> MGSLVREWVGFQQFPAATQEKLIEFFGKLKQKDMNSMTVLVLGKGGVGKSSTVNSLIGEQVVRVSPFQAEGLRPVMVSRTMGGFTINIIDTPGLVEAGYVNHQALELIKGFLVNRTIDVLLYVDRLDVYAVDELDKQVVIAITQTFGKEIWCKTLLVLTHAQFSPPDELSYETFSSKRSDSLLKTIRAGSKMRKQEFEDSAIA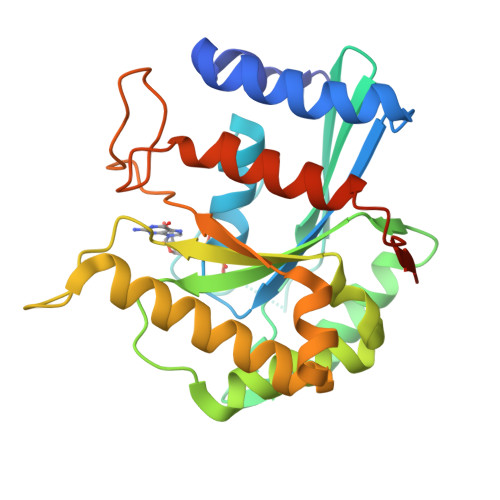VVYAENSGRCSKNDKDEKALPNGEAWIPNLVKAITDVATNQRKAIHVDAAALEHHHHHH>[8x]SNAQVAIITASDSGIGKECALLLAQQGFDIGITWHSDEEGAKDTAREVVSHGVRAEIVQLDLGNLPEGALALEKLIQRLGRIDVLVNNAGAMTKAPFLDMAFDEWRKIFTVDVDGAFLCSQI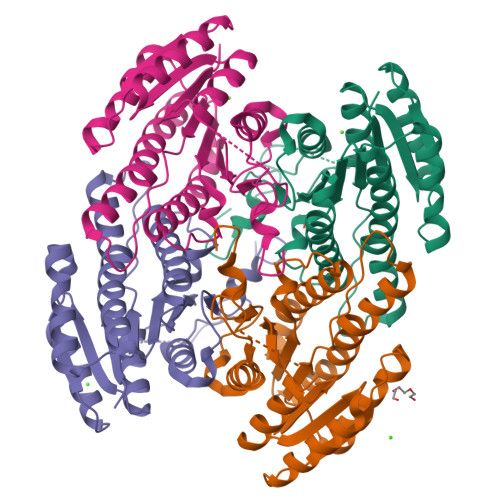AARQMVKQGQGGRIINITSVHEHTPLPDASAYTAAKHALGGLTKAMALELVRHKILVNAVAPGAIATPMNGMDDSDVKPDAEPSIPLRRFGATHEIASLVVWLCSEGANYTTGQSLIVDGGFMLANPQFNPE>[4x]MKHHHHHHMKQNSPLDEENLTQENQDRGTHVDRGLASANVDFAFSLYKQLVLKAPDKNVIFSPLSISTALAFLSLGAHNTTLTEILKGLKFNLTETSEAEIHQSFQHLLRTLNQSSDELQLSMGNAMFVKEQLSLLDRFTEDAKRLYGSEAFATDFQDSAAAKKLINDYVKNG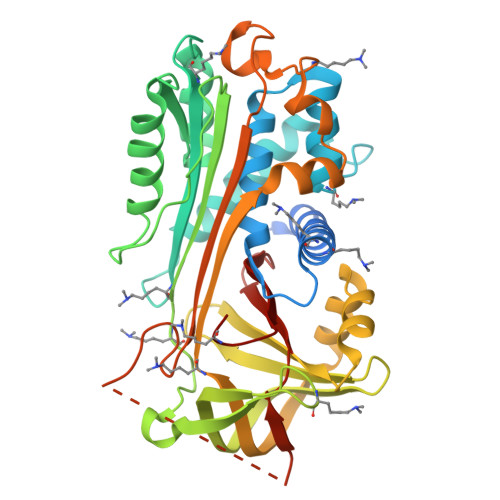TRGKITDLIKDLDSQTMMVLVNYIFFKAKWEMPFDPQDTHQSRFYLSKKKWVMVPMMSLHHLTIPYFRDEELSCTVVQLNYTGNASALFILPDQDKMEEVEAMLSRETLNRWGDSLEFREIGELYLPKFSISRDYNLNDILLQLGIEEAFTSKADLSGITGARNLAVSQVVHKAVLDVFEEGTEASAATAVKITLLSALVETRTIVRFNRPFLMIIVDHFTWSIFFMSKVTNPKQA>[4x]DTMKVINDPIHGHIELHPLLVRIIDTPQFQRLRYIKQLGGGYYVFPGASHNRFEHSLGVGYLAGCLVHALGEKQPELQISERDVLCVQIAGLCRNLGHGPFSHMFDGRFIPLARPEVKWTHEQGSVMMFEHLINSNGIKPVMEQYGLIPEEDICFIKEQIVGPLESPVEDSLWPYKGRPENKSFLYEIVSNKRNGIDVDKWDYFARDCHHLGIQNNFDYKRFIKFARVCEVDNELRICARDKEVGNLYDMFHTRNSLHRRAYQHKVGNIIDTMITDAFLKADDYIEITGAGGKKYRISTAIDDMEAYTKLTDNIFLEILYSTDPKLKDAREILKQIEYRNLFKYVGETQPTGQIKIKREDYESLPKEVASAKPKVLLDVKLKAEDFIVDVINMDYGMQEKNPIDHVSFYCKTAPNRAIRITKNQVSQLLPEKFAEQLIRVYCKKVDRKSLYAARQYFVQWCADRNFTKPQDGDVIAPLITPQKKEWNDSTSVQNPTRLREASK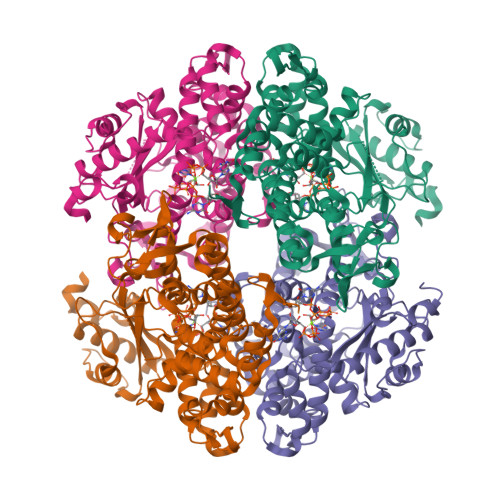SRVQLFKDDPM> GG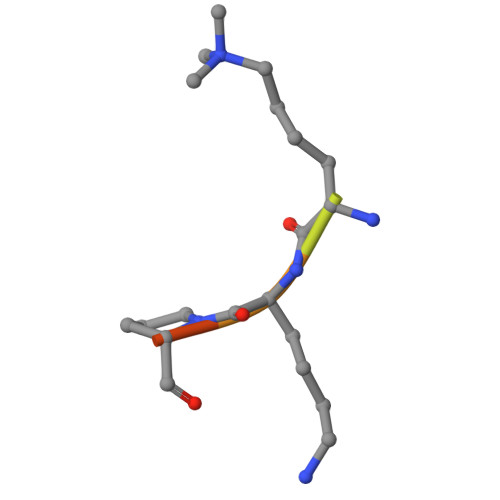VKKPHR>XXXXXXXXXXXXXXXXXXXXXXXXXXXXXXXXXXXXXXXXXXXXXXXXXXXXXXXXXXXXXXXXXXXXXXXXXXXXXXXXXXXXXXXXXXXXXXXXXXXXXXXXXXXXXXXXXXXXXXXXKFLTIPRLEELYNTKQGPTNPMLFHLIRDVKQGNLPPGYKITLIDIGLVIEYLMGGTYRCTYTRKRFRLIYNSLGGNNRRSGRNTSSSTPQLRKSHETFGNRADKKEKMRHNHFIKTAQPYRPKMDASMEEGKKKRTKDEIVDIDDPETKRFPYPLNELLIWACLMKRQVMARFLWQHGEESMAKALVACKIYRSMAYEAKQSDLVDDTSEELKQYSNDFGQLAVELLEQSFRQDETMAMKLLTYELKNWSNSTCLKLAVSSRLRPFVAHTCTQMLLSDMWMGRLNMRKNSWYKVILSILVPPAILMLEYKTKAEMSHIPQSQDAHQMTMEDSENNFHNITEEIPMEVFKEVKILDSSDGKNEMEIHIKSKKLPITRKFYAFYHAPIVKFWFNTLAYLGFLMLYTFVVLVKMEQLPSVQEWIVIAYIFTYAIEKVREVFMSEAGKISQKIKVWFSDYFNVSDTIAIISFFVGFGLRFGAKWNYINAYDNHVFVAGRLIYCLNIIFWYVRLLDFLAVNQQAGPYVMMIGKMVANMFYIVVIMALVLLSFGVPRKAILYPHEEPSWSLAKDIVFHPYWMIFGEVYAYEIDVCANDSTLPTICGPGTWLTPFLQAVYLFVQYIIMVNLLIAFFNNVYLQVKAISNIVWKYQRYHFIMAYHEKPVLPPPLIILSHIVSLFCCVCKRRKKDKTSDGPKLFLTEEDQKKLHDFEEQCVEMYFDEKDDKFNSGSEERIRVTFERVEQMSIQIKEVGDRVNYIKRSLQSLDSQIGHLQDLSALTVDTLKTLTAQKASEASKVHNEITRELSISKHLAQNLIDDVPVRPL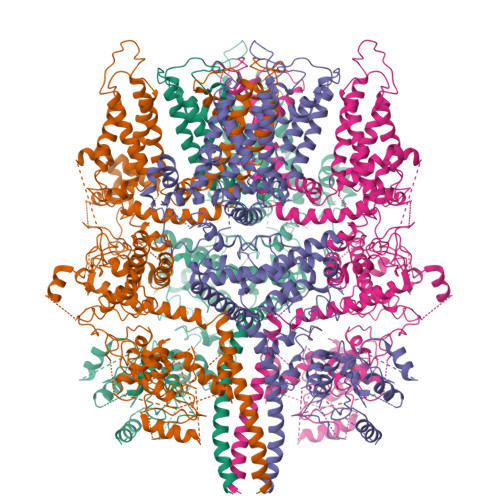WKKPSAVNTLSSS[4x]> SDGYTPE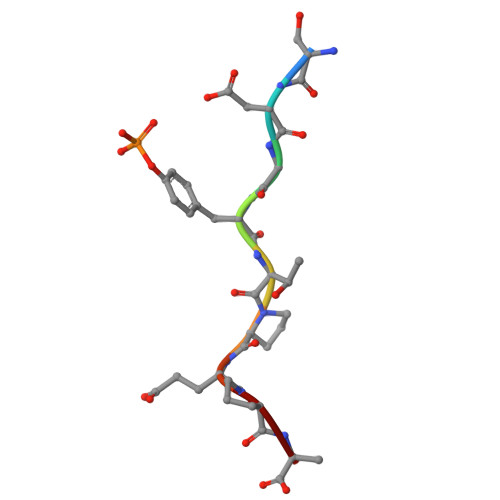PA>MELILNEAEKVFAMHGFLGATLKQIAQNSNVTQALITYYYGTKQNLFMEVYRRGLSDIDKKRQNYLDELKSRPEGYNTYDIVRTYLRPQFEHREGGQAWMHFARLQSRLASEPEEVAVPLRKELYDHTLKAFIHEIMECEGEDDAAAVSWGAVFMVSMILYMLRGVDRIGELTDGHLHAESEDDIVERMTIFITGGINSLKQATQ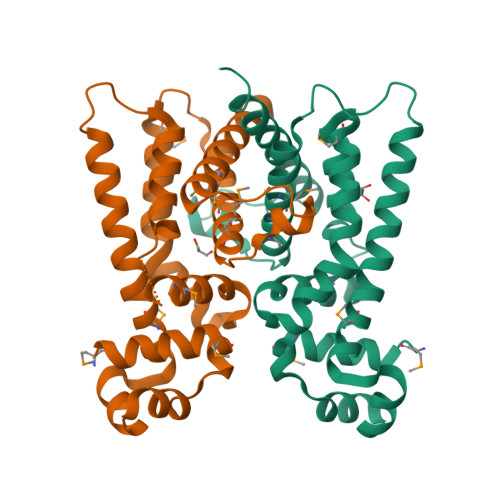DKYK[6x]>KSSNTASVVVLATAPDEATAQDLAAKVLAEKLAAAATLIPGATSLYYWEGKLEQEYVVQMILKTTVSHQQALLEALKSHHPYQTPELLVL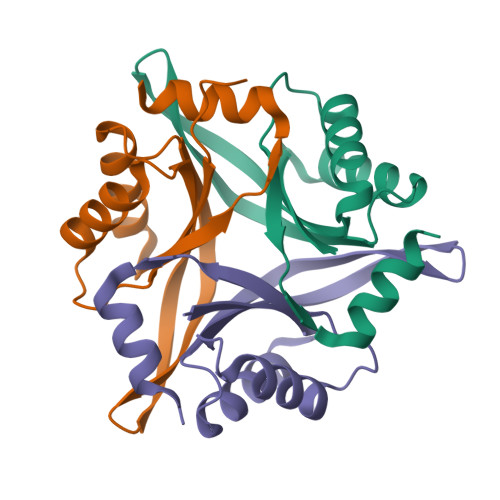PVTHGDTDYLSWLNASLR[6x]> MTHGAVKTYGIRLRVWGDYACFTRPEMKVERVSYDVMPPSAARGILEAIHWKPAIRWIVDRIHVLRPIVFDNVRRNEVSSKIPKPNPATAMRDRKPLYFLVDDGSNRQQRAATLLRNVDYVIEAHFELTDKAGAEDNAGKHLDI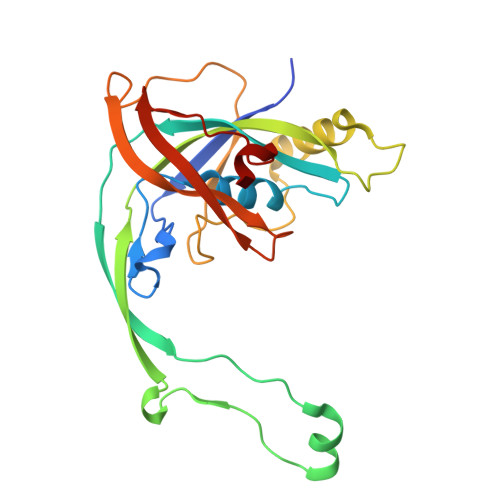FRRRARAGQSFQQPCLGCREFPASFELLEGDVPLSCYAGEKRDLGYMLLDIDFERDMTPLFFKAVMEDDVITPPSRTSPEVRA>[2x]STTLTRQDLNFGQVVADVLCEFLEVAVHLILYVREVYPVGIFQKRKKYNVPVQMSCHPELNQYIQDTLHCVKPLLEKNDVEKVVVVILDKEHRPVEKFVFEITQPPLLSISSDSLLSHVEQLLAAFILKISVCDAVLDHNPPGCTFTVLVHTREAATRNMEKIQVIKDFPWILADEQDVHMHDPRLIPLKTMTSDILKMQLYVEERAHKGS;>[2x]MLSRFIPWFPYDGSKLPLRPKRSPPASREEIMATL

Human Shieldin consists of four subunits, REV7 (also known as MAD2L2 or MAD2B, 211 residues), SHLD1 (205 residues), SHLD2 (835 residues), and SHLD3 (250 residues). As the first identified member of the Shieldin complex, REV7 is composed entirely of a HORMA domain, acting as an interaction module in a broad array of cellular pathways. The Shieldin complex acts as the key downstream effector of 53BP1; it not only binds and shields single-stranded DNA ends but also mediates CST- and Polα-dependent fill-ins of DNA breaks. TRIP13 forms a hexamer to drive the REV7-mediated disassembly of Shieldin in an adenosine triphosphate (ATP)-dependent manner, thereby releasing the DSB DNA ends for resection to promote HDR.

Next, we coexpressed full-length REV7 (R124A mutant) and a fusion protein that contains SHLD3 (residues 35 to 58) and a short stabilizing REV3 sequence (residues 1887 to 1894) (labeled SHLD3s). REV7 Arg-124 was mutated to Ala to improve crystallization. The reported structure of the REV7–REV3 complex implied that the additional short REV3 sequence could potentially enhance complex formation. We then determined the crystal structure of this SHLD3s–REV7 monomer complex at 2.7-Å resolution (X-ray statistics in SI Appendix, Table S1). There are two molecules in the asymmetric unit and the bound SHLD3s can be readily traced into its density in the complex. In contrast to the safety-belt region that binds multiple partners, site-S, which overlays with the REV1-binding site has sufficient complexity, making it ideal for small molecule drug design toward attempts to disrupt the Shieldin/NEHJ pathway. In addition, the site-S interface shares one pocket with the adjacent REV1-binding site and another adjacent one with a pocket identified by the PockDrug server, implying the potential for druggability of site-S. Since disrupting of the REV7–REV1 interaction can inhibit mutagenic translesion synthesis (TLS) and reduce chemoresistance, such a two-component pocket scaffold (adjacent site-S and REV1-binding site) spanning the REV7 surface could represent an attractive future avenue for improving DNA-damaging chemotherapeutics by simultaneously inhibiting error-prone NHEJ and TLS.1,2-DICHLOROETHANE | C2 H4 Cl2 | 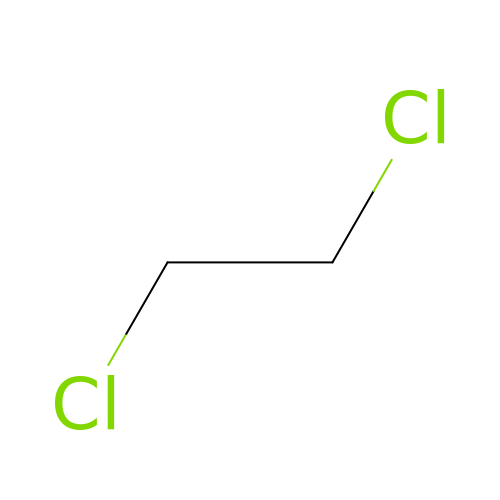WSLDOOZREJYCGB-UHFFFAOYSA-N>MASEALTMIVNLLRSQRPLQEPTVEQMRAGLEAMAQMSPLPADVELTTVDAGGVPGAWVRVPESDPDRVVLYLHGGGYVIGSIRTHRDLAQRIARAARCRVLLIDYRLAPEHPHPAAVEDSTRAYRWLLETGSDPKRMAIAGDSAGGGLTVATLVALRDAGVPLPAAAVCLSPWVDLEGIGESMTTKAAVDPMVQREPLLRMASMYLAGQDPRTPLAAPLYADLRGLPPLLIQVGTAETLL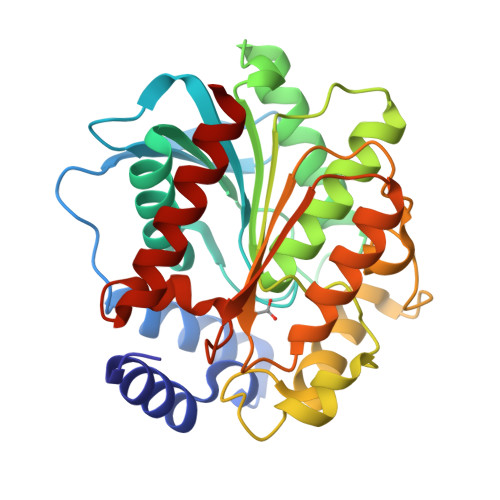DDSVRLAERARAAGVQVTLEPWEDMIHVWQAFAAMLPEGQQAIERIGEFLRQHWQ[2x]3-(carboxycarbonyl)cyclopentane-1-carboxylic acid | C8 H10 O5 | 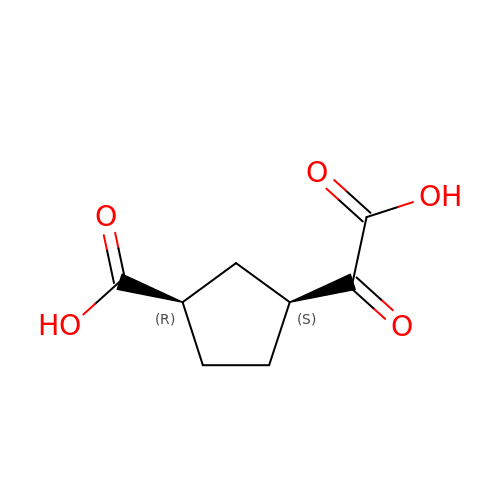BFOGQMGXPDGPQE-CRCLSJGQSA-N>GEDVFEVEKILDMKTEGGKVLYKVRWKGYTSDDDTWEPEIHLEDCKEVLLEFR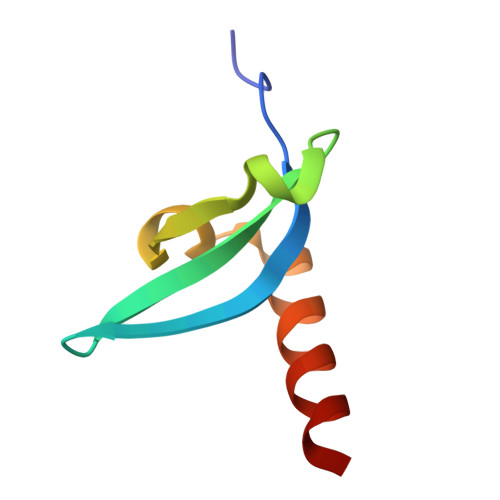KKIAENKAK[2x]>VLKLYGAPMSTCTSRVLTCLHEKNLDFELVPVDLFAGEHKQPPFLAKNPFGQIPALEEDDLTLFESRAITSYIAEKFKGTGYDLIRHENLKEAASVKVWTEVESHRY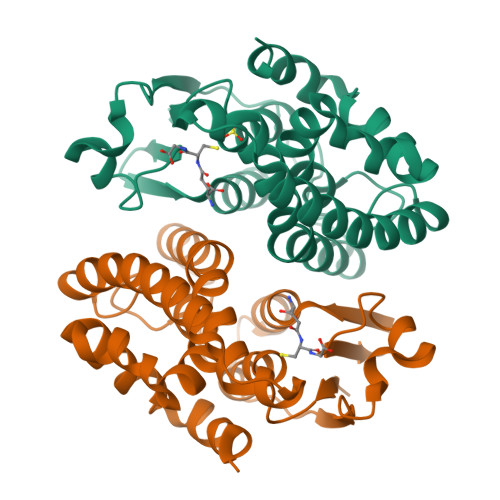NPAIAPIVFQFMVAPLRGNSPDQTIIDDNVEKLGKVLDIYEAKLSSTKYLAGDFYSLADLHHLPYTYYLMKTPAASVVNERPHVKAWWEDISSRPAFKKVAEGMNFVKK[2x]>[2x]RVMYYGKGDVFAYRTYLKPLTGVRTIPESPFSGRDHILFGVNVKISVGGTKLLTSFTKGDNSLVVATDSMKNFIQKHLASYTGTTIEGFLEYVATSFLKKYSHIEKISLIGEEIPFE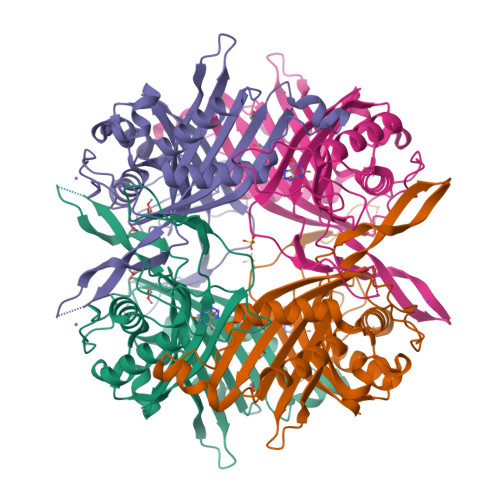TTFAVKNGNRAASELVFKKSRNEYATAYLNMVRNEDNTLNITEQQSGLAGLQLIKVSGNSFVGFIRDEYTTLPEDSNRPLFVYLNIKWKYKNTEDSFGTNPENYVAAEQIRDIATSVFHETETLSIQHLIYLIGRRILERFPQLQEVYFESQNHTWDKIVEEIPESEGKVYTEPRPPYGFQCFTVTQEDLPHENIL[5-(aminomethyl)-1-benzothiophen-2-yl]-tris(oxidanyl)boranuide | C9 H11 B N O3 S 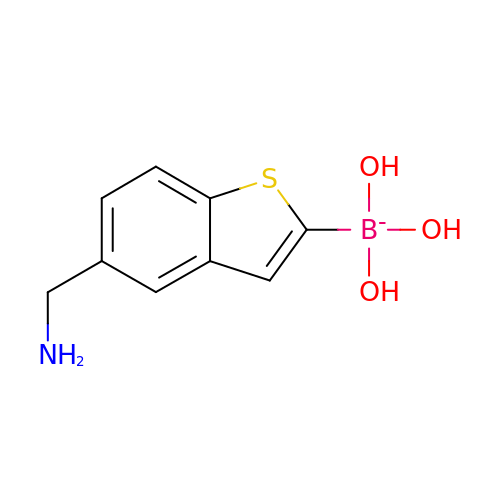| MOEIXULQWWCKOY-UHFFFAOYSA-N> SADIDECESSPCINGVCKNSPGSFICECSSESTLDPTKTICIETIKGTCWQTVIDGRCEININGATLKSQCCSSLGAAWGSPCTLCQVDPICGKGYSRIKGTQCEDIDECEVFPGVCKNGLCVN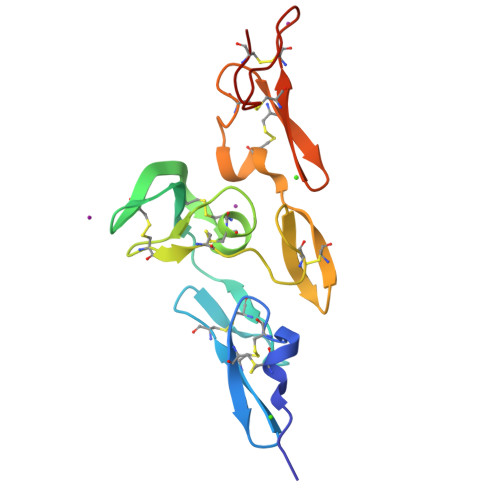TRGSFKCQCPSGMTLDATGRICL> NLAKGKEESLDSDLYAELRCMCIKTTSGIHPKNIQSLEVIGKGTHCNQVEVIATLKDGRKICLDPDAPRIKKIVQKKLAG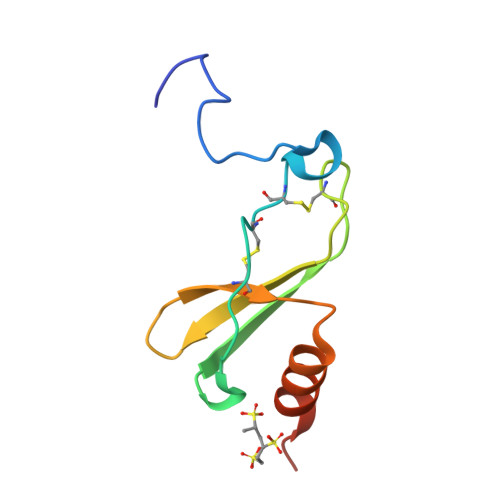DESAD1-(2-chloropyridin-4-yl)-3-phenylurea | C12 H10 Cl N3 O | 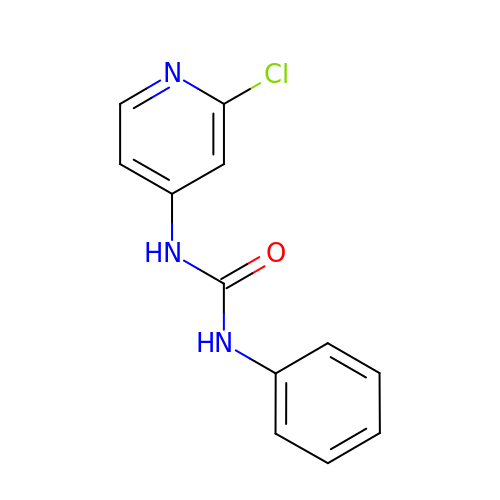GPXLRLUVLMHHIK-UHFFFAOYSA-N> MILDTDYITEDGKPVIRIFKKENGEFKIDYDRNFEPYIYALLKDDSAIEDVKKITAERHGTTVRVVRAEKVKKKFLGRPIEVWKLYFTHPQDQPAIRDKIKEHPAVVDIYEYDIPFAKRYLIDKGLIPMEGDEELKMLAFAIATLYHEGEEFAEGPILMISYADEEGARVITWKNIDLPYVDVVSTEKEMIKRFLKVVKEKDPDVLITYNGDNFDFAYLKKRSEKLGVKFILGREGSEPKIQRMGDRFAVEVKGRIHFDLYPVIRRTINLPTYTLEAVYEAIFGQPKEKVYAEEIAQAWETGEGLERVARYSMEDAKVTYELGKEFFPMEAQLSRLVGQSLWDVSRSSTGNLVEWFLLRKAYERNELAPNKPDERELARRRESYAGGYVKEPERGLWENIVYLDFRSLYPSIIITHNVSPDTLNREGCEEYDVAPQVGHKFCKDFPGFIPSLLGDLLEERQKVKKKMKATIDPIEKKLLDYRQRLIKILANSFYGYYGYAKARWYCKECAESVTAWGRQYLETTIREIEEKFGFKVLYADTDGFFATIPGADAETVKKKAKEFLDYINAKLPGLLELEYEGFYKRGFFVTKKKYAVIDEEDKITTRGLEIVRRDWSEIAKETQARVLEAILKHGDVEEAVRIVKEVTEKLSKYEVPPEKLVIYKQITRDLKDYKATGPHVAVAKRLAARGIKIRPGTVISYIVLKGSGRIGDRAIPFDEFDPAKHKYDAEYYIENQVLPAVERILRAFGYRKEDLRYQKTRQVGLGAWLKPKT

Archaeal DNA polymerases from the B-family (polB) have found essential applications in biotechnology. Variants of the archaeal polymerase from Thermococcus gorgonarius, TgoT, that can either generate HNA from DNA (TgoT_6G12) or DNA from HNA (TgoT_RT521) have been previously identified. In this study, six X-ray structures of DNA and HNA polymerases are reported: (i) three apo- structures of TgoT, TgoT_6G12, and TgoT_RT521-; (ii) two DNA-bound structures of TgoT_6G12 in binary and ternary complexes; and (iii) one DNA-bound structure of TgoT_6G12, which has incorporated two HNA nucleotides. Consistent with all other DNAPs from B-family, TgoT and its variants fold into five distinct structural subdomains.

In addition, another TgoT mutant capable of synthesizing complementary DNA from an HNA template was discovered. This mutant, named TgoT_RT521, is a reverse transcriptase that was engineered de novo. Compared to TgoT, this mutant has only two additional mutations, I521L and E664K. To better understand how the mutations added on TgoT variants impact the structure of the polymerase, the X-ray structures of the apo form of TgoT, replicative polymerase TgoT_6G12, and reverse transcriptase TgoT_RT521 were solved by crystallography. Crystals were obtained for the three polymerases and diffracted at 2.4, 3.1, and 2.35 Å, respectively. Comparison of TgoT_6G12 with TgoT_RT521 structures shows a strong similarity between the two polymerases (r.m.s. deviation for Cα atoms: 0.6 Å). The final apo TgoT_6G12 and TgoT_RT521 structures contained flexible segments in the thumb subdomains. Slight movements in the finger domain (r.m.s. deviation for Cα atoms: 1.18 Å for TgoT_RT521 and 1.1 Å for TgoT_6G12) and in the exonuclease domain (r.m.s. deviation for Cα atoms: 0.8 Å for TgoT_RT521 and 1.0 Å for TgoT_6G12) were observed for both mutants. On the contrary, larger rigid-body movements in the palm domains (r.m.s. deviation for Cα atoms: 2.7 Å for TgoT_RT521 and 2.3 Å for TgoT_6G12) were observed. For example, between amino acids 619 to 660, for TgoT_RT521, the r.m.s. deviation for Cα is 9.4 Å and between amino acids 619 and 650 for TgoT_6G12, it is 7.9 Å.> MSTSQTKNVSIDTIKEFMYQVLLKVGSDEENARMVRDTLIAADLRGMDTHGIQRFKTVYIDRIKKGMINPTAKPSIIRETSTTCVLDGNNGFGHVNGTIGMKMAIEKAKKYGMGMVVVRNSTHFGIAGYYSLLAAQEGCIGICGTNARSSVAATFGDEPILGTNPLAIGIPSDEAFPYCFDGATSISPTGRFEKYVRMGKTVDKSWASMKGGKPIEDPKELLENYPKGKAYLHPLGGSDEVSGSHKGYCLSEFVEIMSSCLSIANFLNHIEEEKEKSGKFSLGHFFIAINVECFRDLNEFKKNVGDINRTLRNTDKLPGHDRIYTAGEKEYETEQKRRKFGD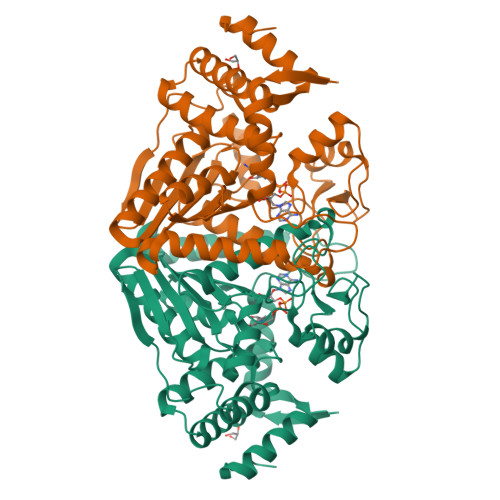DLPLVTINEMKELSSFYNVPLPF> GMNSNFSYPALGVDGISSQISPIRDVWSTNLQQEMNLIMSLIERYPVVSMDTEFPGVVARPLGVFKSSDDYHYQTLRANVDSLKIIQIGLALSDEEGNAPVEACTWQFNFTFNLQDDMYAPESIELLTKSGIDFKKHQEVGIEPADFAELLIGSG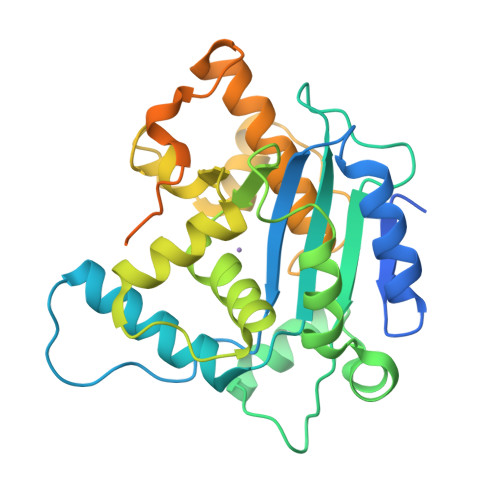LVLQEEVTWITFHSGYDFAYLLKAMTQIPLPAEYEEFYKILCIYFPKNYDIKYIMKSVLNNSKGLQDIADDLQIHRIGPQHQAGSDALLTARIFFEIRSRYFDGSIDSRMLNQLYGLGSTGSVLWHNNSSTPQIQFRDLPGAHPSPTPSNAGIPTTLTNTSSAPNFANSTFRFPPRVV> MGLNDIFEAQKIEWHEMGNTSSERAALERHGGHKTPRRDSSG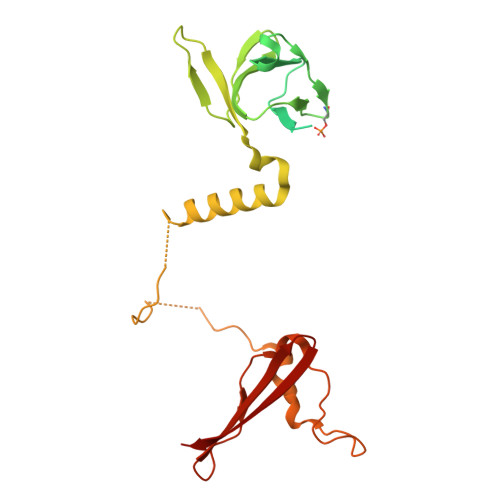GTKDGDRPKILMDSPEDADLFHSEEIKAPEKEEFLAWQHDLEVNDKAPAQARPTVFRWTGGGKEVYLSGSFNNWSKLPLTRSHNNFVAILDLPEGEHQYKFFVDGQWTHDPSEPIVTSQLGTVNNIIQVKKTDFEVFDALMVDSQKCSDVSELSSSPPGPYHQEPYVCKPEERFRAPPILPPHLLQVILNKDTGISCDPALLPEPNHVMLNHLYALSIKDGVMVLSATHRYKKKYVTTLLYKPI>MVSANGDLHLPISNEQCMPENNGSLGFEAPTPDRFDRDRLFSVVSRGVPEELTGLLEYLRWNSKYLTDSAYTEGSTGKTCLMKAVLNLQDGVNACIMPLLQIDKDSGNPKPLVNAQCTDEFYQGHSALHIAIEKRSLQCVKLLVENGADVHLRACGRFFQKHQGTCFYFGELPLSLAACTKQWDVVTYLLENPHQPASLEATDSLGNTVLHALVMIADNSPENSALVIHMYDGLLQMGARLCPTVQLEEISNHQGLTPLKLAAKEGKIEIFRHILQREFSGPYQPLSRKFTEWCYGPVRVSLYDLSSVDSWEKNSVLEIIAFHCKSPNRHRMVVLEPLNKLLQEKWDRLVSRFFFNFACYLVYMFIFTVVAYHQPSLDQPAIPSSKATFGESMLLLGHILILLGGIYLLLGQLWYFWRRRLFIWISFMDSYFEILFLLQALLTVLSQVLRFMETEWYLPLLVLSLVLGWLNLLYYTRGFQHTGIYSVMIQKVILRDLLRFLLVYLVFLFGFAVALVSLSREARSPKAPEDNNSTVTEQPTVGQEEEPAP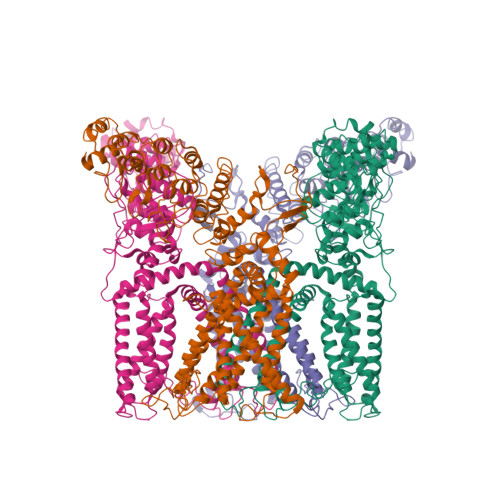YRSILDASLELFKFTIGMGELAFQEQLRFRGVVLLLLLAYVLLTYVLLLNMLIALMSETVNHVADNSWSIWKLQKAISVLEMENGYWWCRRKKHREGRLLKVGTRGDGTPDERWCFRVEEVNWAAWEKTLPTLSEDPTETSQVAPASTOP[4x]> SPKYTKSVLKKGDKTNFPKKGDVVHC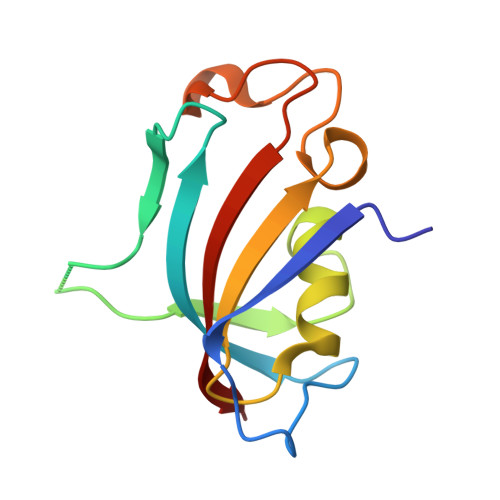WYTGTLQDGTVFDTNIQTSAKKKKNAKPLSFKVGVGKVIRGWDEALLTMSKGEKARLEIEPEWAYGKKGQPDAKIPPNAKLTFEVELVDID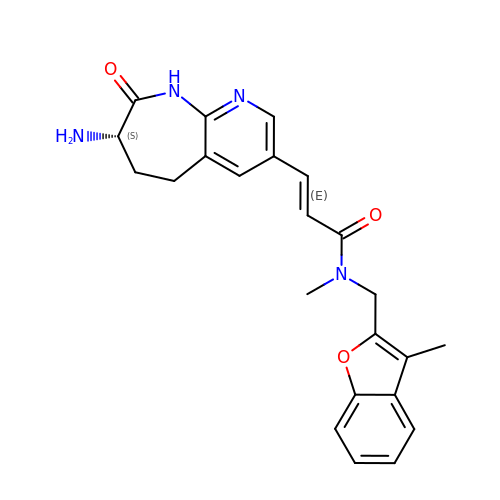(2E)-3-[(7S)-7-amino-8-oxo-6,7,8,9-tetrahydro-5H-pyrido[2,3-b]azepin-3-yl]-N-methyl-N-[(3-methyl-1-benzofuran-2-yl)methyl]prop-2-enamide | C23 H24 N4 O3 | ZWQNEFFHBSGFHV-HKMNZKMDSA-N> AMPFEIEVLLPGEISPAETSALQKCEGKIITFSTLRHRASLVDIALSSYYINGAPPDTLSLLEAYRMRFAAVITRVIPGKLLAHAIGVGTPTPGLFIQNTSPVDLCNGDYICLLPPVFGSADEIRLDSVGLEIVFPLTIPQTLMREIIAKVVARAVERTAADVICYNGRRYELETNLQHRDGSDAAIRTLVL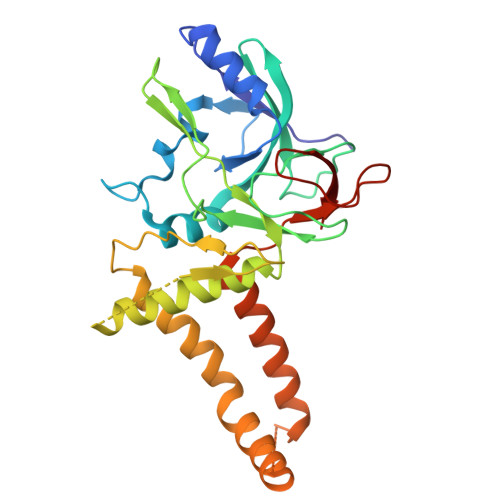NLMFSINEGTTLILTLITRLLRFPIYEAISSWISTSSRLGDTLGTRAILRVCVFDGPSTVHPGDRTAVIQV> APRQHLLSLTRRAQKHRLRELKIQVKEFADKEEGGDVKAVCLTLFLLALRARNEHRQADELEAIMQGRGSGLQPAVCLAIRVNTFLSCSQYHKMYRTVKAITGRQIFQPLHALRNAEKVLLPGYHPFEWQPPLKNVSSRTDVGIIDGLSGLASSVDEYPVDTIAKRFRYDSALVSALMDMEEDILEGMRSQDLDDYLNGPFTVVVKESCDGMGDVSEKHGSGPAVPEKAVRFSFTVMRITIEHGSQNVKVFEEPKPNSELCCKPLCLMLADESDHETLTAILSPLIAEREAMKSSELTLEMGGIPRTFKFIFRGTGYDEKLVREVEGLEASGSVYICTLCDTTRLEASQNLVFHSITRSHAENLQRYEVWRSNPYHESVEELRDRVKGVSAKPFIETVPSIDALHCDIGNAAEFYKIFQLEIGEVYKHPNASKEERKRWQATLDKHLRKRMNLKPIMRMNGNFARKLMTQETVDAVCELIPSEERHEALRELMDLYLKMKPVWRSSCPAKECPESLCQYSFNSQRFAELLSTKFKYRYEGKITNYFHKTLAHVPEIIERDGSIGAWASEGN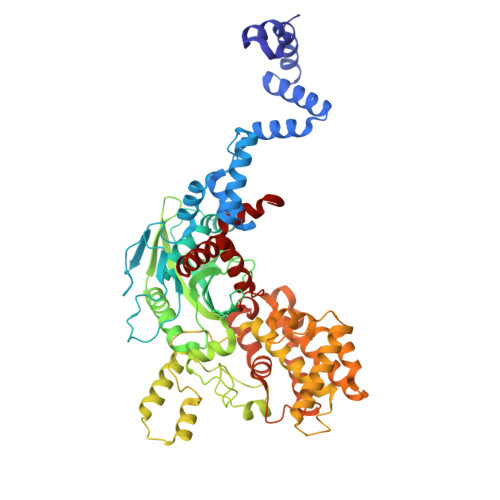ESGNKLFRRFRKMNARQSKCYEMEDVLKHHWLYTSKYLQKFMNAHNA>MDIHSHQQALDAYENVLEHLREKHIRITETRKAIISYMIQSTEHPSADKIYRDLQPNFPNMSLATVYNNLKVLVDEGFVSELKISNDLTTYYDFMGHQHVNVVCEICGKIADFMDVDVMDIAKEAHEQTGYKVTRIPVIAYGICPDCQAKDQPDFLEHHHHHH[2x]

PerR is the peroxide response transcriptional regulator that controls genes expression under oxidative stress and it is required for full virulence. PerR belongs to the Fur (ferric uptake regulator) super family known to be dimeric, metal-binding regulators. PerR has been identified as a repressor that blocks transcription initiation by binding to a specific site (the per box) in the promoter region of target genes. Similar to Fur and Fur-like proteins, the GAS PerR monomer can be divided into an N-terminal DNA-binding domain (residues 1–94) and a C-terminal dimerization domain (residues 98–149 in chain A and residues 98–157 in chain B).

We solved the crystal structure of PerR to 1.6 Å resolution by three-wavelength MAD phasing, using zinc as the anomalous scatter. The structure represents the assembly of a homodimer in the asymmetric unit. Each subunit consists of six α-helices (α1 to α6) and six β-strands (β1 to β6). No exogenous zinc was added during the process of protein purification or crystallization, suggesting that an endogenous zinc is normally bound at the regulatory site, coordinated with residues His4, His6, Asn15, His19, His97, His99 in a pseudo octahedral geometry. The results showed that mutations in the residues of the zinc-finger motif or of the regulatory site, abolished the DNA binding ability of PerR, but not the control residues H44A and N101A. The overall conformation of our GAS PerR-Zn-Zn structure is substantially different from that of the B. subtilis PerR-Zn-Mn structure, which displays a DNA-binding-competent conformation. Our recombinant GAS PerR protein with a DNA-binding activity, however, exhibits a DNA-binding-incompetent conformation similar to the B. subtilis apo-PerR-Zn structure. SAXS studies show that the crystallographic structure of GAS PerR is indeed consistent with its solution formation. Alanine substitution of any of Y67A, N69A and K83A also reduced but did not completely eliminate DNA binding. This study strongly suggests that residues Arg21, Arg26, Arg31, Asn69, Tyr67, Asn68, Lys71 and Lys83, located on the positively charged patch, are involved in PerR interaction with DNA. In the model, the DNA-binding interface is contributed from two adjacent PerR homodimers in tetrameric assembly. This distinct DNA-binding feature explains that PerR dimer alone is in the DNA-binding-incompetent conformation.> HXEGXFTSDVSSYLEGQAAKEF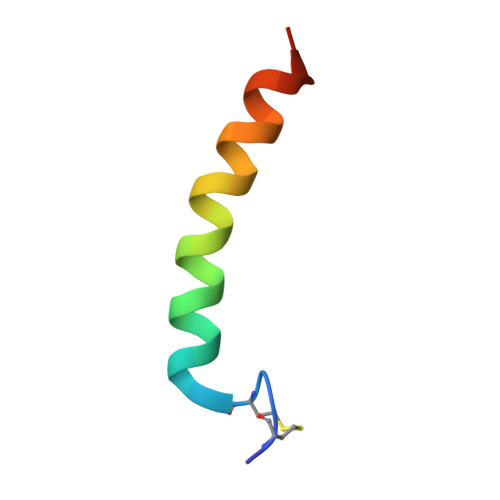IAWLVKGRG>[6x]PESPSKLASAIQKAHEEGICGIRSVTRLENLMWKQITPELNHILTENEVKLTIMTGDIKGIMQAGKRSLRPQPTELKYSWKAWGKAKMLSTELHNHTFLIDGPETAECPNTNRAWNSLEVEDYGFGVFTTNIWL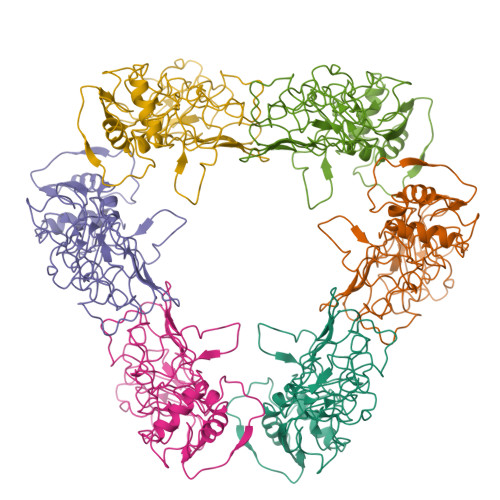KLKERQDVFCDSKLMSAAIKDNRAVHADMGYWIESALNDTWKIEKASFIEVKSCHWPKSHTLWSNGVLESEMIIPKNFAGPVSQHNYRPGYHTQTAGPWHLGRLEMDFDFCEGTTVVVTEDCGNRGPSLRTTTASGKLITEWCCRSCTLPPLRYRGEDGCWYGMEIRPLKEK> MQSYSRRWFLGAGATTLISAAGLTACGSGSGSGGSGGTITAMVYGDDAVKVQDKAASRFNASAEAKKANAKVKMERIPASDYPAKLRTAMGSPNAPDIFFNWGGGSIKAYKEAGQLVDLTDVIKSDEVLSTGFLPSVVAAGSLDGHEYGIPMRGMQPVLLFYNKSVFAEHKLTPPTTWDQLLDNVAKL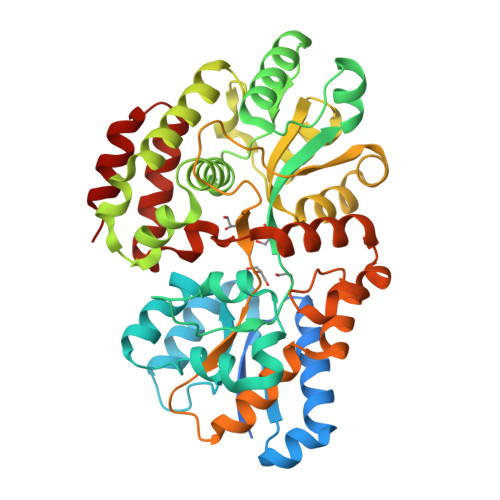KKAGVTPFALGGVEIWPELMWLEYLVDRIGGPQVFDKIRNGDASGWGDPAVLKAAQTVKQLVDEGAFGKGFSSVSYNNGGAPALLAKGKAGMHLMGSWEYSTQLGKFPDFAKKDLGWCAFPSFEGGAGDIRNVVGNPCNYWSVNARTGNKDGAIAFLRDCASEAYTKDLIDNGDVPTTTIAENMLDSSPNPEFAKFQYQLVQKAPNFTLSWDQAVDPDWQQPMLTEINKLFVGKSSPEQFVSALKGLK> PQFEKIEGRMIRILYLLVKPESMSHEQFRKECVVHFQMSAGMPGLH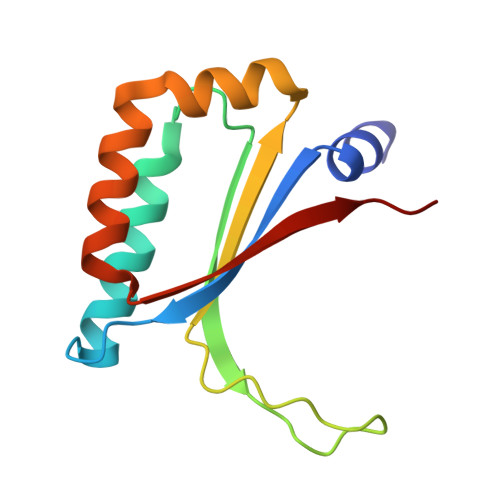KYEVRLVAGNPTDTHVPYLDVGRIDAIGECWFASEEQYQVYMESDIRKAWFEHGKYFIGQLKPFVTEELV>MEAAHSKSTEECLAYFGVSETTGLTPDQVKRHLEKYGHNELPAEEGKSLWELVIEQFEDLLVRILLLAACISFVLAWFEEGEETITAFVEPFVILLILIANAIVGVWQERNAENAIEALKEYEPEMGKVYRADRKSVQRIKARDIVPGDIVEVAVGDKVPADIRILSIKSTTLRVDQSILTGESVSVIKHTEPVPDPRAVNQDKKNMLFSGTNIAAGKALGIVATTGVSTEIGKIRDQMAATEQDKTPLQQKLDEFGEQLSKVISLICVAVWLINIGHFNDPVHGGSWIRGAIYYFKIAVALAVAAIPEGLPAVITTCLALGTRRMAKKNAIVRSLPSVETLGCTSVICSDKTGTLTTNQMSVCKMFIIDKVDGDFCSLNEFSITGSTYAPEGEVLKNDKPIRSGQFDGLVELATICALCNDSSLDFNETKGVYEKVGEATETALTTLVEKMNVFNTEVRNLSKVERANACNSVIRQLMKKEFTLEFSRDRKSMSVYCSPAKSSRAAVGNKMFVKGAPEGVIDRCNYVRVGTTRVPMTGPVKEKILSVIKEWGTGRDTLRCLALATRDTPPKREEMVLDDSSRFMEYETDLTFVGVVGMLDPPRKEVMGSIQLCRDAGIRVIMITGDNKGTAIAICRRIGIFGENEEVADRAYTGREFDDLPLAEQREACRRACCFARVEPSHKSKIVEYLQSYDEITAMTGDGVNDAPALKKAEIGIAMGSGTAVAKTASEMVLADDNFSTIVAAVEEGRAIYNN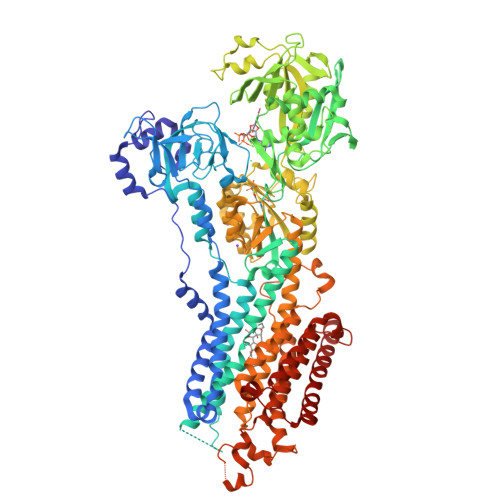MKQFIRYLISSNVGEVVCIFLTAALGLPEALIPVQLLWVNLVTDGLPATALGFNPPDLDIMDRPPRSPKEPLISGWLFFRYMAIGGYVGAATVGAAAWWFMYAEDGPGVTYHQLTHFMQCTEDHPHFEGLDCEIFEAPEPMTMALSVLVTIEMCNALNSLSENQSLMRMPPWVNIWLLGSICLSMSLHFLILYVDPLPMIFKLKALDLTQWLMVLKISLPVIGLDEILKFIARNYLEG[2x]> FRRKEDLDPPLALLPLKGLREAAALLEEALRQGKRIRVHGDYDADGLTGTAILVRGLAALGADVHPFIPHRLEEGYGVLMERVPEHLEASDLFLTVDCGITNH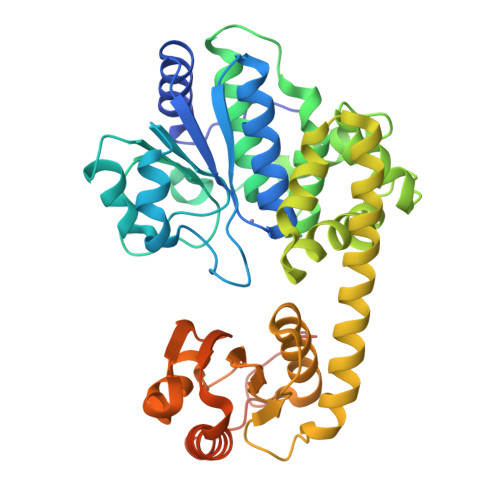AELRELLENGVEVIVTDHHTPGKTPPPGLVVHPALTPDLKEKPTGAGVAFLLLWALHERLGLPPPLEYADLAAVGTIADVAPLWGWNRALVKEGLARIPASSWVGLRLLAEAVGYTGKAVEVAFRIAPRINAASRLGEAEKALRLLLTDDAAEAQALVGELHRLNARRQTLEEAMLRKLLPQADPEAKAIVLLDPEGHPGVMGIVASRILEATLRPVFLVAQGKGTVRSLAPISAVEALRSAEDLLLRYGGHKEAAGFAMDEALFPAFKARVEAYAARFPDPVREVALLDLLPEPGLLPQVFRELALLEPYGEGNPEPLFL>SMRKTIERLLNSELSSNSIA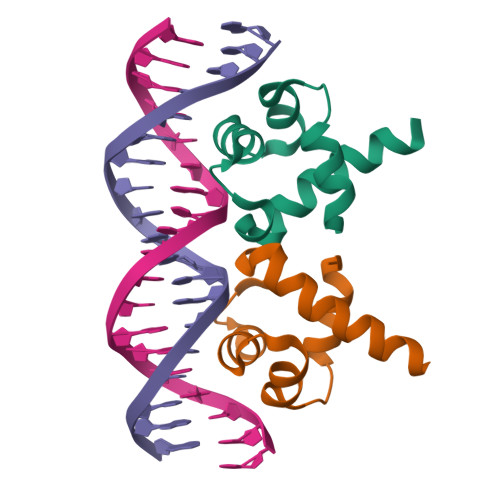VRTGVSQAVISKLRNGKKELGNLTLNSAEKLFEYQKEMEKVDT[4x]>[2x]MDRRFPPFSPFFNHGRFFDDVDFDRHMIRPYWADQTMLTGHRVGDAIDVVNNDQEYNVSVDVSQFEPE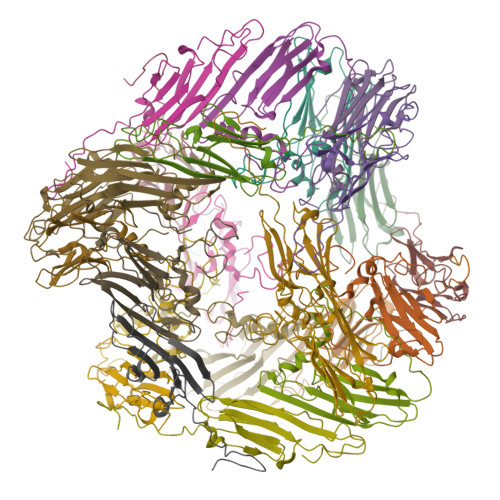ELKVNIVDNQLIIEGKHNEKTDKYGQVERHFVRKYNLPTGVRPEQIKSELSNNGVLTVKYEKNQEQQPKSIPITIVPKRN6-AMINO-4-[2-(4-METHYLPHENYL)ETHYL]-1,7-DIHYDRO-8H-IMIDAZO[4,5-G]QUINAZOLIN-8-ONE 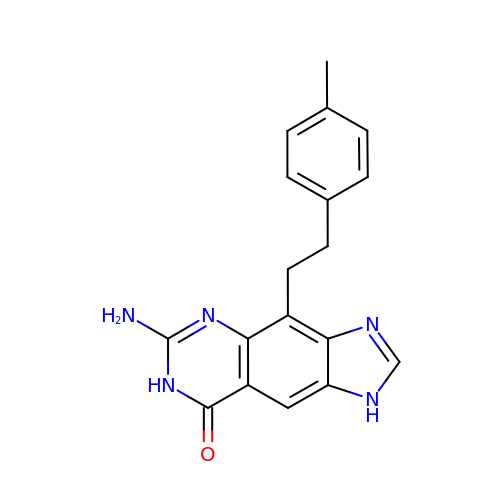| C18 H17 N5 O | SPVJRTJUEVXOMS-UHFFFAOYSA-N> MELKNSISDYTEAEFVQLLKEI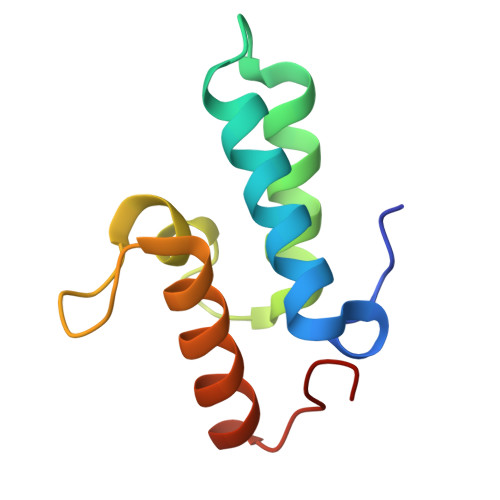EKENVAATDDVLDVLLEHFVKITEHPDGTDLIYYPSDNRDDSPEGIVKEIKEWRAANGKPGFKQG>[3x]SDLIPAPPLSKVP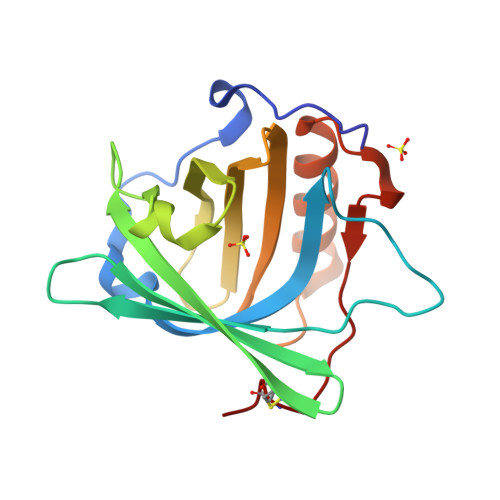LQQNFQDNQFQGKWYVVGLAGNAILREDKDPQKMYATIYELKEDKSYNVTSVLFRKKKCDYWIRTFVPGSQPGEFTLGNIKSYPGLTSYLVRVVSTNYNQHAMVFFKKVSQNREYFKITLYGRTKELTSELKENFIRFSKSLGLPENHIVFPVPIDQCIDG> SWGFIYKTLKS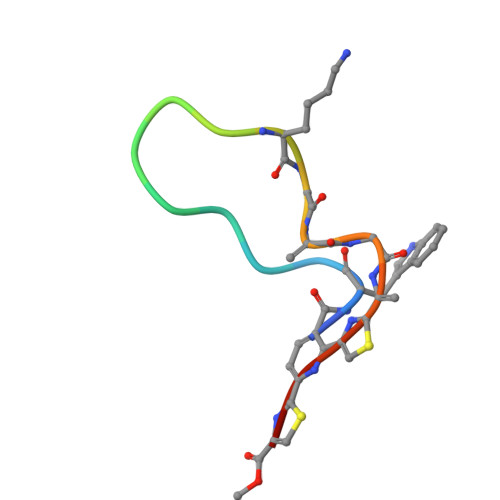SGSCSCX> GMTDMNPDIEKDQTSDEVTVETTSVFRADFLSELDAPAQAGTESAVSGVEGLPPGSALLVVKRGPNAGSRFLLDQAITSAGRHPDSD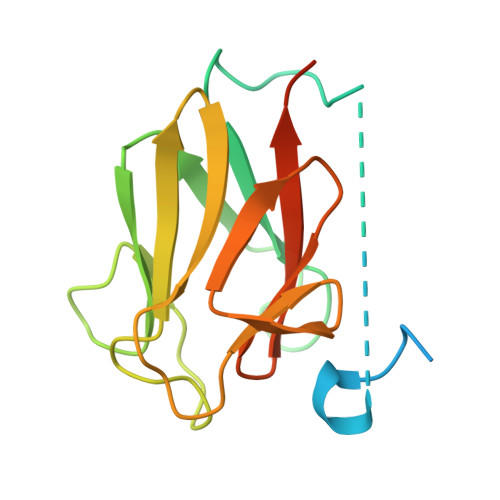IFLDDVTVSRRHAEFRLENNEFNVVDVGSLNGTYVNREPVDSAVLANGDEVQIGKFRLVFLTGPKQGEDDGSTGGP> MSTAKAPTLPASIFRAYDIRGVVGDTLTAETAYWIGRAIGSESLARGEPCVAVGRDGRLSGPELVKQLIQGLVDCGCQVSDVGMVPTPVL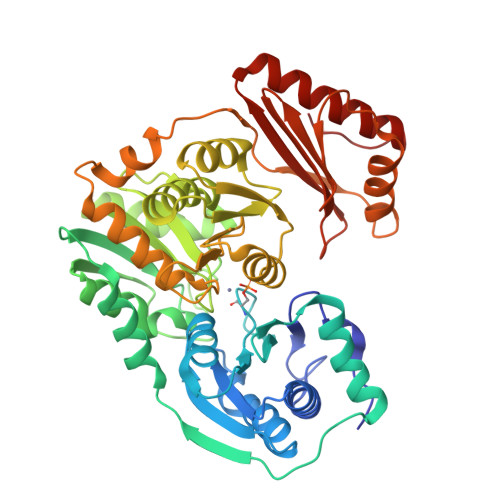YYAANVLEGKSGVMLTGSHNPPDYNGFKIVVAGETLANEQIQALRERIEKNDLASGVGSVEQVDILPRYFKQIRDDIAMAKPMKVVVDCGNGVAGVIAPQLIEALGCSVIPLYCEVDGNFPNHHPDPGKPENLKDLIAKVKAENADLGLAFDGDGDRVGVVTNTGTIIYPDRLLMLFAKDVVSRNPGADIIFDVKCTRRLIALISGYGGRPVMWKTGHSLIKKKMKETGALLAGEMSGHVFFKERWFGFDDGIYSAARLLEILSQDQRDSEHVFSAFGSDISTPEINITVTEDSKFAIIEALQRDAQWGEGNITTLDGVRVDYPKGWGLVRASNTTPVLVLRFEADTEEELERIKTVFRNQLKAVDSSLPVPF> MIIGNCLILKDFSSEPFWGAVEIENGTIKRVLQGEVKVDLDLSGKLVMPALFNTHTHAPMTLLRGVAEDLSFEEWLFSKVLPIEDRLTEKMAYYGTILAQMEMARHGIAGFVDMYFHEEWIAKAVRDFGMRALLTRGLVDSNGDDGGRLEENLKLYNEWNGFEGRI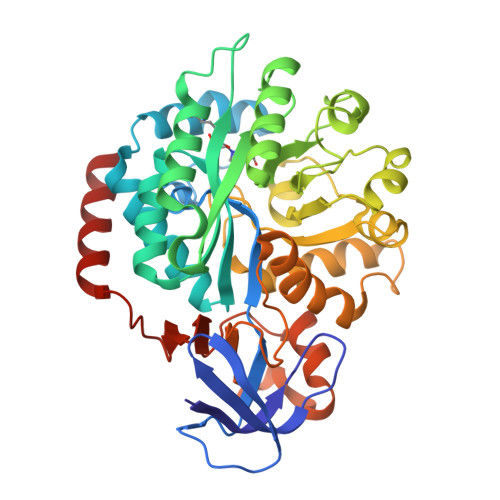FVGFGPHSPYLCSEEYLKRVFDTAKSLNAPVTIHLYETSKEEYDLEDILNIGLKEVKTIAAHCVHLPERYFGVLKDIPFFVSHNPASNLKLGNGIAPVQRMIEHGMKVTLGTDGAASNNSLNLFFEMRLASLLQKAQNPRNLDVNTCLKMVTYDGAQAMGFKSGKIEEGWNADLVVIDLDLPEMFPVQNIKNHLVHAFSGEVFATMVAGKWIYFDGEYPTIDSEEVKRELARIEKELYSS>TGGRNSIRYSELAPLFDTTRVYLVDNKST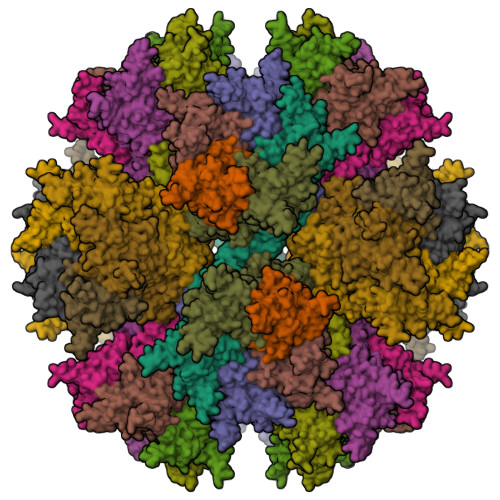DVASLNYQNDHSNFLTTVIQNNDYSPGEASTQTINLDDRSHWGGDLKTILHTNMPNVNEFMFTNKFKARVMVSRSLTKDKQVELKYEWVEFTLPEGNYSETMTIDLMNNAIVEHYLKVGRQNGVLESDIGVKFDTRNFRLGFDPVTGLVMPGVYTNEAFHPDIILLPGCGVDFTHSRLSNLLGIRKRQPFQEGFRITYDDLEGGNIPALLDVDAYQASLKDDTEQGGDGAGGGNNSGSGAEENSNAAAAAMQPVEDMNDHAIRGDTFATRAEEKRAEAEAAAEAAAPAAQPEVEKPQLKPVIKPLTEDSKKRSYNLISNDSTFTQYRSWYLAYNYGDPQTGIRSWTLLCTPDVTCGSEQVYWSLPDMMQDPVTFRSTSQISNFPVVGAELLPVHSKSFYNDQAVYSQLIRQFTSLTHVFNRFPENQILARPPAPTITTVSENVPALTDHGTLPLRNSIGGVQRVTITDARRRTCPYVYKALGIVSPRVLSSRTF[15x]>MATLKASSLRALKLMHLATSANDDDTDENVIALCHQAKTPVGNTDAIFIYPRFIPIARKTLKEQGTPEIRICTSTNFPHGNDDIDIALAETRAAIAYGADSVAVVFPYRALMAGNEQVGFDLVKACKEACAAAN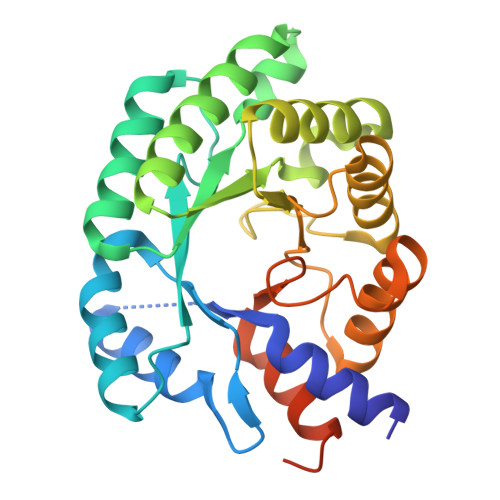VLLAVIIETGELKDEALIRKASEISIKAGADNIVTSTGKVAVGATPESARIMMEVIRDMGVEKTVGFIPVGGVRTAEDAQKYLAIADELFGADWADARHYAFGASASLLASLLKALGHGDGKSASSYGSLEHHHHHH[2x]> GAQVSRQNVGTHSTQNSVSNGSSLNYFNINYFKDAASNGASKLEFTQDPSKFTD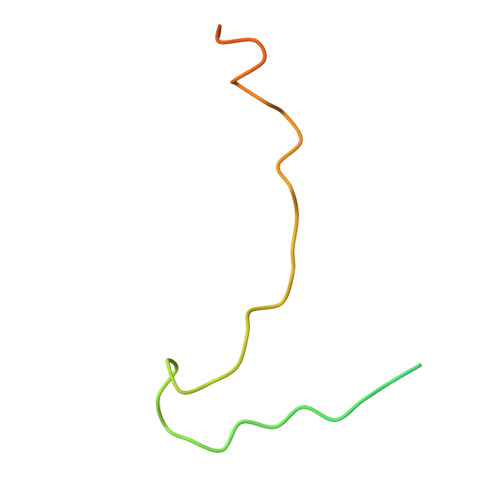PVKDVLEKGIPTLQ> SRWMEPYFDPSTPRNVTALMGKSAYLSCRVRNLANKTVSWIRHRDIHILTVGSYTYTSDQRFQATHHQDTEDWTLQIKWAQKRDAGMYECQISTQPVRSYFVRLNVVVPH;> SRAFQPEFVESISNVSVAVGRDATFTCHVRHLGGYRVGWLKADTKAIQAIHENVITHNPRVTVSHLDQNTWNLHIKAVSEEDRGGYMCQLNTDPMKSQIGFLDVVI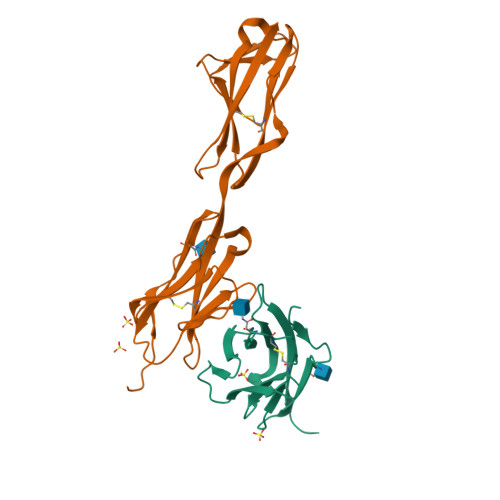PPDFISEDTSSDVIVPEGSSVRLTCRARGYPEPIVTWRREDGNEIVLKDNVGTKTLAPSFRGEVLKLSKISRNEMGSYLCIASNGVPPSVSKRISLSIHH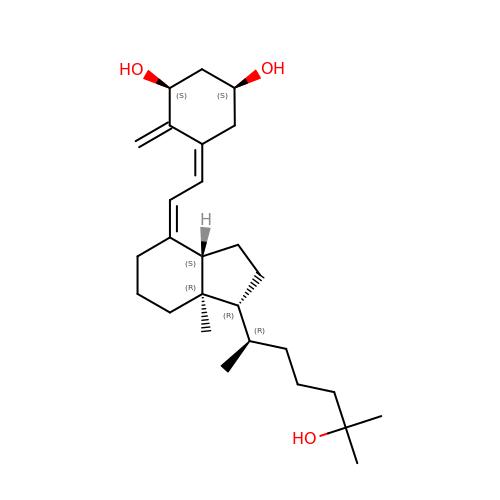(1S,3S,5Z,7E,14beta,17alpha)-9,10-secocholesta-5,7,10-triene-1,3,25-triol | C27 H44 O3 | GMRQFYUYWCNGIN-GNVXBELXSA-N Classical Zn2+-dependent deac(et)ylases play fundamental regulatory roles in life and are well characterized in eukaryotes regarding their structures, substrates and physiological roles. Structurally, these enzymes are composed of a central eight-stranded parallel β-sheet flanked by α-helices on each site, known as the α/β-arginase/deacetylase fold. All active site residues were conserved, as shown by the multiple sequence alignment and the structural alignment, suggesting a general acid/base catalytic mechanism for the bacterial enzymes as described for the eukaryotic counterparts. These enzymes mediate catalysis using a penta-coordinated catalytic Zn2+ ion coordinated by two aspartates and a histidine (KpHdaH (1b): Asp181, Asp269, His183).

RwDmhA (1b) is a dimethoate amidohydrolase, i.e. the substrate specificity changed from acetylated lysine side chains to a small molecule phosphorothionate. For RwDmhA (1b) we identified an all-trans octanoic acid in the substrate binding tunnel coordinating the active site Zn2+ ion with its carboxylate moiety. We did neither supply the acetate nor the octanoic acid in the crystallization condition, which might therefore originate from protein production and the activity of the enzymes in E. coli. For RwDmhA (1b) and RsPrpH (1b) we discovered a hydrophobic 22-LFL-24/32-LYF-34 motif in the L1-loop lining the substrate binding tunnel, the sequence 98-GHLAP-102/107-GMLAP-111 as well as the sequence 342-MAEAW-346/352-MFALW−356 in the C-terminal α-helix lining the active site rim. These residues form a hydrophobic active site and contribute to the binding of the observed octanoic acid in RwDmhA (1b). Only for RwDmhA (1b) and RsPrpH (1b), which evolved toward non-protein substrates, the second proline is substituted for an Ala suggesting this position being important for substrate specificity to accommodate the product. For RwDmhA (1b), we discovered it being an active lysine deacylase, which might suggest that this 1b enzyme is capable to act as lysine deacylase additionally to the reported dimethoate hydrolase activity. For RwDmhA (1b), we identified an all-trans-octanoic acid in the crystal structure, suggesting RwDmhA (1b) being capable of releasing this fatty acid upon deacylation from their substrate. As a consequence, we propose RwDmhA (1b) having additional yet undefined substrates apart from dimethoate.

>[4x]MAHHHHHHVGTMARTGFYTDERTFWHATGMQALFLPVGDWVQPPNGTAGADTPDSKRRLLNLAHASGLIRKLTLPEAIPATVEDVCRVHPRDYIDRFKATSDAGGGDLGHLAPFSKGGYEIAMLSCGLAIAAVDDVLSGKVDNAYALCRPAGHHCLADTPMGFCLLANIPIAIEAAKARHGISRVAVVDWDVHHGNGTQSIFYDRADVLTISIHQDRCFPPGYSGAEDRGEGAGLGYNLNVPLPAGAGHDAYVQAFDDIVVPALDDFKPDLIIVASGLDANSVDPLARMLLHSESYRLLTQKMLDAAARLCGGKLVVVHEGGYAEAYVPFCGHALLEALSGERTAVVDPVLEMAEAWQPGPEAAAFHRQWIDRLVADLGK> MSATKSIVGEALEYVNIGLSHFLALPLAQRISLIIIIPFIYNIVWQLLYSLRKDRPPLVFYWIPWVGSAVVYGMKPYEFFEECQKKYGDIFSFVLLGRVMTVYLGPKGHEFVFNAKLADVSAEAAYAHLTTPVFGKGVIHDCPNSRLMEQKKFVKGALTKEAFKSYVPLIAEEVYKYFRDSKNFRLNERTTGTIDVMVTQPEMTIFTASRSLLGKEMRAKLDTDFAYLYSDLDKGFTPINFVFPNLPLEHYRKRDHAQKAISGTYMSLIKERRKNNDIQDRDLIDSLMK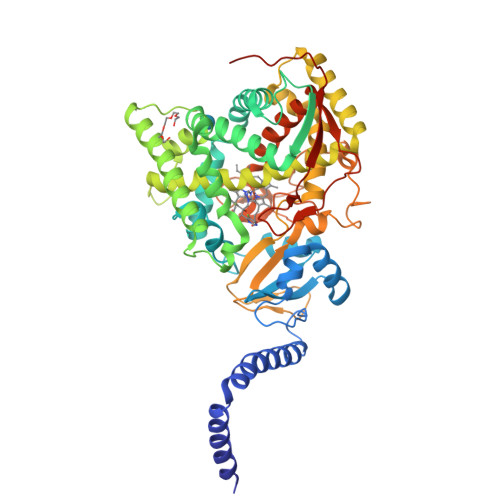NSTYKDGVKMTDQEIANLLIGVLMGGQHTSAATSAWILLHLAERPDVQQELYEEQMRVLDGGKKELTYDLLQEMPLLNQTIKETLRMHHPLHSLFRKVMKDMHVPNTSYVIPAGYHVLVSPGYTHLRDEYFPNAHQFNIHRWNNDSASSYSVGEEVDYGFGAISKGVSSPYLPFGGGRHRCIGEHFAYCQLGVLMSIFIRTLKWHYPEGKTVPPPDFTSMVTLPTGPAKIIWEKRNPEQKIGGRHHHHHH> ATSDDWKSKAIYQLLTDRFGRADDSTSNCSNLSNYCGGTYEGITKHLDYISGMGFDAIWISPIPKNSDGGYHGYWATDFYQLNSNFGDESQLKALIQAAHERDMYVMLDVVANHAGPTSNGYSGYTFGDASLYHPKCTIDYNDQTSIEQCWVADELPDIDTEN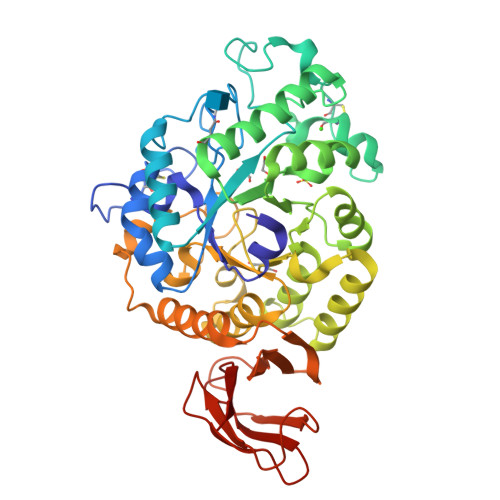SDNVAILNDIVSGWVGNYSFDGIRIDTVKHIRKDFWTGYAEAAGVFATGEVFNGDPAYVGPYQKYLPSLINYPMYYALNDVFVSKSKGFSRISEMLGSNRNAFEDTSVLTTFVDNHDNPRFLNSQSDKALFKNALTYVLLGEGIPIVYYGSEQGFSGGADPANREVLWTTNYDTSSDLYQFIKTVNSVRMKSNKAVYMDIYVGDNAYAFKHGDALVVLNNYGSGSTNQVSFSVSGKFDSGASLMDIVSNITTTVSSDGTVTFNLKDGLPAIFTSA;> ATSDDWKSKAIYQLLTDRFGRADDSTSNCSNLSNYCGGTYEGITKHLDYISGMGFDAIWISPIPKNSDGGYHGYWATDFYQLNSNFGDESQLKALIQAAHERDMYVMLDVVANHAGPTSDGYSGYTFGDASLYHPKCTIDYNDQTSIEQCWVADELPDIDTENSDNVAILNDIVSGWVGNYSFDGIRIDTVKHIRKDFWTGYAEAAGVFATGEVFNGDPAYVGPYQKYLPSLINYPMYYALNDVFVSKSKGFSRISEMLGSNRNAFEDTSVLTTFVDNHDNPRFLNSQSDKALFKNALTYVLLGEGIPIVYYGSEQGFSGGADPANREVLWTTNYDTSSDLYQFIKTVNSVRMKSNKAVYMDIYVGDNAYAFKHGDALVVLNNYGSGSTNQVSFSVSGKFDSGASLMDIVSNITTTVSSDGTVTFNLKDGLPAIFTSA>PHEELQYLRQLREILCRGSDRLDRTGIGTLSLFGMQARYSLRDHFPLLTTKRVFWRGVVQELLWFLKGSTDSRELSRTGVKIWDKNGSREFLAGRGLAHRREGDLGPVYGFQWRHFGAAYVDADADYTGQGFDQLSYIVDLIKNNPHDRRIIMCAWNPADLSLMALPPCHLLCQFYVADGELSCQLYQRSGDMGLGVPFNIASYSLLTYMLAHVTGLRPGEFIHTLGDAHIYKTHIEPLRLQLTRTPRPFPRLEILRSVSSMEEFTPDDFRLVDYCPHPTIRME[2x]

TS is an essential enzyme for DNA replication. It catalyzes the transfer of a methylene group from the cofactor 5,10-methylenetetrahydrofolate (mTHF) to its substrate 2′-deoxyuridine-5′-monophosphate (dUMP) and produces thymidine-5′-monophosphate (dTMP) and dihydrofolate (DHF). KSHV encodes functional thymidylate synthase (kTS), which shares 70% sequence identity with hTS. The overall structure of kTS was found to have a similar structural conformation to hTS, except minor differences in ligand binding site and conformational variations in some amino acids.

In apo kTS, phosphate molecules occupied the dUMP binding site. In addition, a dual conformation was observed for the sulfhydryl group of catalytic Cys219, as shown in the electron density map of apo kTS. Arg200’ residue in the apo kTS structure was rotated approximately 145° to the opposite direction of the phosphate group and was not observed to interact with dUMP. For kTS, the Arg74 residue in apo and ternary complex did not interact with in dUMP, whereas the corresponding Arg residue in other TS structures was shown to interact with the phosphate group of dUMP. In apo and ternary kTS structures, the C-terminal region (residues Glu334–Val337) was not assigned due to the lack of an electron density map.The best characterized and most clinically important efflux system in N. gonorrhoeae is the MtrCDE tripartite multidrug efflux system, which belongs to the hydrophobic and amphiphilic efflux resistance-nodulation-cell division (HAE-RND) family. The membrane fusion protein MtrC, containing 412 amino acids, bridges MtrD and MtrE to form the tripartite efflux complex MtrCDE. This powerful efflux complex spans the entire cell envelope of N. gonorrhoeae and mediates the export of hydrophobic antimicrobial agents, such as antibiotics, nonionic detergents, antibacterial peptides, bile salts and gonadal steroidal hormones.

For the MtrCDE tripartite efflux system, MtrD is a large proton-motive-force (PMF)-dependent inner membrane HAE-RND efflux pump composed of 1,067 amino acids. It appears that the opening and closing of the MtrE channel may be induced by the change in conformation of the MtrC membrane fusion protein, which propagates the progressive motion of the MtrD multidrug efflux pump within the transport cycle to the MtrE channel. As MtrD is a PMF-dependent pump, this may imply that active proton translocation within the MtrD inner membrane efflux pump provides the energy to open and close the MtrE outer membrane channel.

> MAKFFIDRPIFAWVISIFIIAAGIFGIKSLPVSQYPSVAAPTITLHAIYPGASAQVMEGSVLSVIERNMNGVEGLDYMSTSADSSGSGSVSLTFTPDTDENLAQVEVQNKLSEVLSTLPATVQQYGVTVSKARSNFLMIVMLSSDVQSTEEMNDYAQRNVVPELQRIEGVGQVRLFGAQRAMRIWVDPKKLQNYNLSFADVGSALSAQNIQISAGSIGSLPAVRGQTVTATVTAQGQLGTAEEFGNVILRANTDGSNIYLKDVAKVGLGMEDYSSSTRLNGVNTTGMAVMLSNSGNAMATAKAVKERLAVLEKYFPQGMSWKTPYDTSKFVEISIEKVIHTLIEAMVLVFVVMYLFLQNIRYTLIPTIVVPISLLGGFAFISYMGMSINVLTMFAMILVIGIVVDDAIVVVENVERIMAGEGLPPKEATKKAMGQISGAVIGITAVLISVFVPLAMFSGAAGNIYKQFALTMASSIAFSAFLALTLTPALCATMLKTIPKGHHEEKKGFFGWFNKKFDSWTHGYEGRVAKVLRKTFRMMVVYIGLAVVGVFLFMRLPTSFLPTEDQGFVMVSVQLPAGATKERTDATLAQVTQLAKSIPEIENIITVSGFSFSGSGQNMAMGFAIFKDWNERTASGSDAVAVAGKLTGMMMGTLKDGFGIAVVPPPILELGNGSGLSINLQDRNNTGHTALLAKRNELIQKMRASGLFDPSTVRAGGLEDSPQLKIDINRAAAAAQGISFADIRTALASALSSSYVSDFPNQGRLQRVMVQADEDARMQPADILNLTVPNKSGVAVPLSTIATVSWENGTEQSVRFNGYPSMKLSASPATGVSTGQAMEAVQKMVDELGGGYSFEWGGQSSEEAKGGSQTLILYGLAVAAVFLVLAALYESWSIPLAVILVIPLGLIGAAAGVTGRNLFEGLLGSVPSFANDIYFQVGFVTVMGLSAKNAILIIEFAKDLQAQGKSAVEAALEAARLRFRPIIMTSFAFILGVVPLYIAAGASSASQRAIGTTVFWGMLVGTLLSVFLVPLFYVVVRKFFKETAHEHEMAVRHASK> MHHHHHHMSVYTVKQMARLSGVSVRALHHYDAIGLLKPRAVGANGYRYYDRQDLLRLQQILFH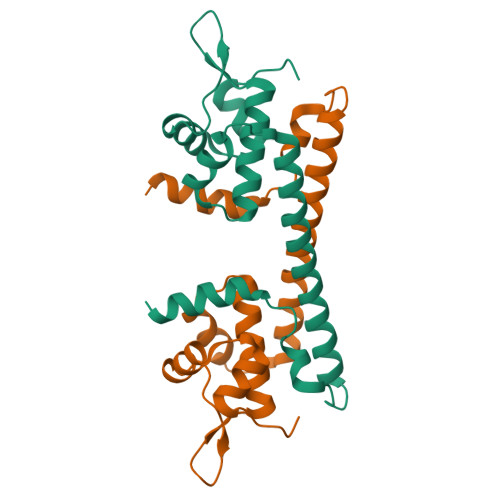RALETPLKDIQAALDQPGFDLAAALRAQRERLAAQAERYARLVDVVDRTLADLEGDETMDDKHLFEGFDPEKQARHEAWLVEHYGDEATRRIADAKAGMKSWGKKDWSQFQEEAKAIEHDLAKALTQGLPVDSAPVTAIMRRHWAWVGRSWNREPTPDAFAGLGHLYQANPEFTARYEAIAPGLTEYFSEAMRAFARGR>[3x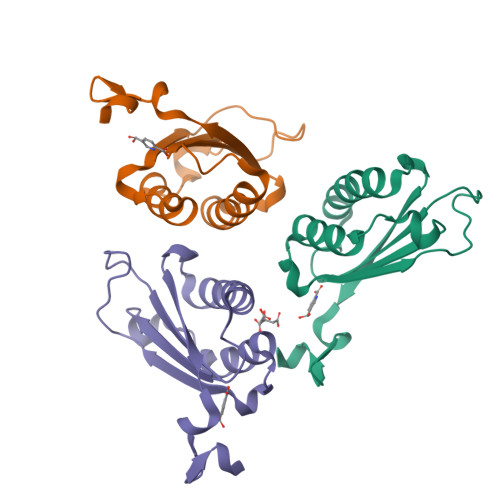]MPFLELDTNLPANRVPAGLEKRLCAAAASILGKPADRVNVTVRPGLAMALSGSTEPCAQLSISSIGVVGTAEDNRSHSAHFFEFLTKELALGQDRILIRFFPLESWQIGKIGTVMTFL> GKRQFVNEWAAEIPGGPEAASAIAEELGYDLLGQIGSLENHYLFKHKNHPARSAASAFHITKRLSDDDRVIWAEQQYEKERSKR

Proprotein convertases (PCs), including furin and PC1/3 among nine mammalian homologues, mediate the maturation of numerous secreted substrates by proteolytic cleavage. The zymogens of the furin-like PCs share a multidomain architecture comprising an N-terminal pro-domain, a subtilisin-like catalytic domain, and a P-domain (also called HomoB-domain). Activation of furin is triggered by two sequential autocatalytic cleavages and subsequent release of the prodomain. In this work, we investigate the structural and functional basis of PC-activation to engineer prodomain-based PC-inhibitors.

M2 includes three Arg-Ala mutations to prepare a stable prodomain:furin complex. To verify the conformation of the secondary cleavage site loop, we solved the structure of isolated M2 at pH 8.3 and refined it to 1.3 Å resolution. Indeed, this region showed the same conformation in isolated and furin-bound M2. For the structure of isolated M2 only the positions of Cα, Cβ, and Cɣ of the side chain of Arg78 were build. Gln30 was modeled in two conformations. In the isolated structure of M2 and in the complex structure with furin, we found an unusual interaction of the His72 side chain with the amide nitrogen atoms of Asn74 and His75. The donor-hydrogen-acceptor angle towards Asn74 (169°) indicates a stronger contribution than the less optimal angle towards His72 (155°) as determined from the isolated M2 structure. The distances between the amide nitrogen atoms and Nδ of His72 are in both cases 3.1°Å. His72 can only act as a hydrogen bond acceptor in a deprotonated state. Thus, protonation of His72 at pH 6.0 will change a productive interaction to an unfavored contact, probably destabilizing the conformation of the secondary cleavage site loop.>[3x]MRRFGSKFASGLASRCALACPLASAATAPAGASTTSSTSSAQKSFFKTTEMIGYVHSIDGTIATLIPAPGNPGVAYNTIIQIQVSPTTFAAGLVFNLEKDGRIGIILMDNITEVQSGQKVMATGQLLHIPVGAGVLGKVVNPLGHEVPVGLVTRSRRLLDSTLGKVDTGAPNIVSRSPVNYNLLTGFKAVDTMIPIGRGQRELIVGDRQTGKTSIAVSTIINQVRINQQILSKNAVISIYVSIGQRCSNVARIHRLLQSYGALRYTTVMAATAAEPAGLQYLAPYAGVTMGEYFMNRGRHCLCVYDDLSKQAVAYRQISLLLRRPPGREAYPGDVFYLHSRLLERAAMLSPGKGGGSVTALPIVETLSNDVTAYIVTNVISITDGQIYLDTKLFTGGQRPAVNIGLSVSRVGSSAQNAAMKGVAGKLKGILAEYRKLAADSVGGQQVQTIPMIRGARFVALFNQKQPSYFMNAIVSLYACLNGYLDDVKVQYVKFYEYLLVHRDLGIMYGTAKNKFFYMYVQELNYLIRFFTLNSPILHGELEEMLKQHTHLFLQHYQSKMNAIKSEKDVKALKNLLYSCKRAV;>MLTRFRSAVLRGAVSITGARAASTAPVADHKGRVGHVSQVIGAVVDVHFADGVPPVLTALDVVDKLGRDEPLTLEIVQHLDAHTGRCIAMQTTDLLKLKAKVVSTGGNISVPVGRETLGRIFNVLGDAIDQRGPVGEKLRMPIHAVAPKLADQAAEDAVLTT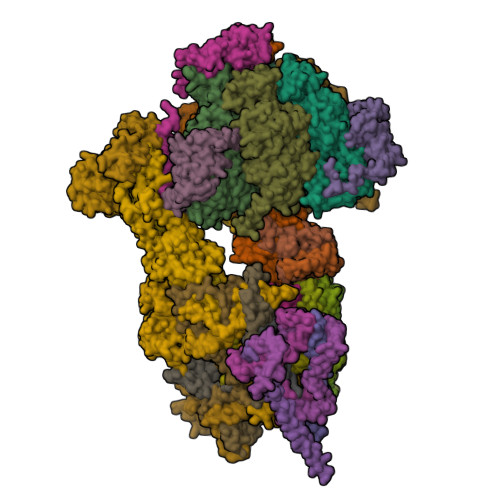GIKVIDLILPYCKGGKIGLFGGAGVGKTVIIMELINNVAKGHGGFSVFAGVGERTREGTDLYLEMMQSKVIDLKGESKCVLVYGQMNEPPGARARVAQSALTMAEYFRDVEGQDVLLFIDNIFRFTQANSEVSALLGRIPAAVGYQPTLAEDLGQLQERITSTTKGSITSVQAVYVPADDITDPAPATTFSHLDATTVLDRAVAESGIYPAVNPLECASRIMDPDVISVDHYNVAQDVVQMLTKYRELQDIIAVLGIDELSEEDKLIVDRARKLVKFLSQPFQVAEVFTGMTGHYVQLDDTIDSFSGLLMGTYDQVPEMAFYMVGGINSVLEKAKKMAEEAAELEKMRRARVAQASS[3x];> MSGKLRLYKEKLEGYNRFYSIVKTIKMVTLAKYRAAQGRIRTRDFSLRYTELAFSKPQASRDAVVAAKNALVYIPITTNRGSCGALNSNIVRCIDSVVSSKMVLMPVGKRGIDSFSKLYPDEFRYGIINDMKESMHFGYATFVIENAYEVSKDADRYQVIFNRFVSAGVQRNAVYNIPSYEKWKEDLADAASSDNQKNRYLFANALQNEEEQLIRDFFDFHAALAVLNAVGENELSEQAARLVAVEGQLTNISSLQQRTSSLYNKTRQFGITAALIEILSAMSSLEGNAMKGVRRNKFWEGAVTK;> MFRTFGRRLVSCTLPLLQSAPHDLPEGFEFMEHKVVNKDIHAPHENLETLRLTLTRQDEFLLREEPVKCVTVTGTNGEYGIYPGHAYKIVQLNPSPLTVEYTDGTTKKYFVSGGFAHINNEGSCDVNTVECTLLDDLDLAIAEKELAAQQAALGSAKDDKAKSVVEIRISVIEAVIAALKHH;> MIRRSCALLSSSWRDHGISYLKYLNVCTETLHSTVKESRRAKYERWSKPCYTAQRPDGAGGQETIDKVPIHTKDY;>[3x]MMRRVYSPVFCSVAAARFAATSAAKKYDLFGYEVDTNTAPWIEKIKKCKYYDEAGEVLVNMNVSNCPPDIATYNATLQCIYQSPSKQSTPVDNESKFCAMMDLLEEMQHRNRLKPNEESWTWVMKECVKSGQFRLGYCIQQVMETECKGCPADLVKANEANAQKAKTEGKEHPGHLSQQAGLFDVKVE;>MSAKAAPKTLHQVRNVAYFFAAWLGVQKGYIEKSANDRLWVEHQRKVRQQNVERQQALDSIKLMQQGVRATTPGQLEGVPAELQQLAEAFTK[2x];>[2x]MSSTKCAVACKIMTPLCNAASKVQARSAKKLAALTDAGIQKTISEHNANGTDAAVSSTKRYLAEQRQLFHYRVVRFFDECHYIISGEYFAQYTKVNLIWDLRFLTKLVVLFLIGTVLGRQSIFPPIDPDSPLVEALVTKVNPNY;> MFRRLSSSARAVVAARFYTPPEGLKKLYASDFENSKYPLNIVPSDSVLFAKFLYKAAEEKGNFDNILSDFQKIAAAASKLPIFWERTAVVEKIPEFKQLSEPTFFTLVWMQNNGMLELIQEVAEVYETFVNAKQKKAVAKIFVAPGGEKNVEEARRVAEELHKGLKELADYTLVLKTVVDRTIVKGFAVELAGQYVNKAEGQQKQAGRADEVDYTNLPAPKPQKTVWDDNIETEVLRKYLDGLSQYDMEEAKYGV;>MMRRLALQSSIRRATPFATPLVASTKALNPMCSAITIREASTVAISVQGLHYVGTGLAAIALAGVGLGIGTIFGNLLVACARQPNLTKMLFNYAILGFALTEAIGLFALMLAFLMLFS[10x];> MFLFFFCDLFWLRLLLCMYYCVWSRLCFIVYFNCLMLIFDFLLFCLFDLYLFVGLCLFLLLWFMLFNLYSLILYYCITYLNLYLLFCIVFLLYIAFLFLFCFLCDFFLFNNLLVGDSFMDVFFIRFLLCFLECFSLLCRCLSTFLRLFCNLLSSHFLLLMFFDFFYFIFVFFFYGVFCYWFILFIFVFCFCLLFYVFLYLLDLFAAILQLFIFCNMILQLIMDFLLFLLFV;> MLRRLGANVSNMARPMNKYAVTVSPRRHLEPMSTWYLASWAMVWYYAFFFWMPMVWTDIMVPSFVYNKLPVIHFLQEKRAEQKLRRVLDETYTEWTEELDQAHVTDAITRSLNI;> MRRVSSPNITIQSVRWISGVSPLLYFPPTTTSTTNREDQINKNTNIAIQMIKRYKGEVPPHYTRKSSATIEQVEKEIDALLGGAEKLRKTSTDDQPMDKLTLMERCLRHALWSYHKEEGRYDFDQIGRWVVYTPEDEVKLAQLKREVEAKEKLAALRKRREEEGLPGGPVPRINWPQEYSSFIDREPVVAKRIRYDTLASTTLERDEKQIESTLQQYRRASQDKRLDDLVDLLERFKPVLAREAIMQRLTIKHLEGQLGVWRYMDWCPEVRDRAELEVDITGWQWWSPLEERRLLPVRLRSVNEVREIMSKTQAKKSAEAAERNPIVTQTSTGDNARDRLLKEVLALQARINQRDEVEPSQTEQKKKAHH;> MQGSWSVLKKNCSNFFPGLLAFAQQTQEAYGIWLRIYNRQQKYGPTDFVEQSETFSPDYHKRFHSQDKNMWVDKELCTEVSQKEVARLMTYKLDMWRMAHCAGALLATGGYAIPFGLFWLANDTWVPSSFNLTGEELRAWREAQDLYRYRSAPSYLTDTKWHFDFHAYPWNETQERAWDDLFEKNDVRRDPKVVRPAAEMYDGFIKFELIRRKSLRHLCRSMNIPTFPMLARLCNGTRVRDYWNLAWCEDYMVITQRLHESMTDEELYDYAWRRYLAPYDKNLNREQLMERVEDYFEFLGPDFVAHGKAPNLVILTNYVLGYYNDPAYLEGDISELDKNDYDHLASWGKDAFLRRLEFENGPLRDQVEAHTQRLLAERAAIAKGDNAAAVEGRHTA;> MVLFSTYRSSRLVSKEFLHGPVMRFRALGEYYFQRAWNGTLNWALPGEYRLYAVMIPFIYFYHRWHNDHTLDRDHVEKAMIMRWGGTLEDVRKLSAKDQLRVRCFTDIEKLYSAYGPKDTYLQPPGDTLPGKDFYRKAGGAQAHH;> MSKQLTFISAGATAAVLQSASAIVSKVAGGRVQTKTAKEAGRHAVVVGPETPIGVHTAVTEVPKSAQDPLFSGVSTVVVRAVLPRAAPDSVQLRDALDVYASAGIDTKEEVRSATEAFKKSAEVAVGKAKAKGVKRIVLVVKQASKHNCINELFKKISTETIESAGLTTEVVGTAAVANQLIVNPESLGVVLLNDVAATEQIELAFAGVVGGVSRVYHTVEGGKISAGHSFKSVALAVAQELRELGLSSEADKVEAAASKNPRAVVSAL;> MRRTFISFSAASAAAAAPVTSTKMQTLHKLLTGEVSFKNKAPVKDCNIVHQFGENWATELSAYAKTLPAEQQKIIVRQIARVKLTRYTVAELAAYCGDGPALLDETARAANIEQGVAFVKAKGVEAFEKYVAEESTNANWKPEEAKKFIEDVKAKAK;> MVYTRWKCDRLPVFQLKLFTQEYPMHAAVGIFTIIFLWKHMSHCSEETERKYGWWAGYPYWRDPIARRNETKYKQMIINNDVDITHPKWTGCSVEQLEELSRVV;> MTKYELKMQYFDEWMIRWRKFQTESDWEIEKGRQWWRRFNMAVSGALFCGLVLYTSGTATLKRQYGLPHFFDIGVDGQAKETMLKTLTSRWRYTPQGYGRVLITGVPTYILFVTLEHYRERRRMQQYLQQNTVFGEQMRRLLSTGKIEEYLPVNIKATLPASQQAIYNY;> MLRRSSAALIRRTPVRHSGGELFVRPKLEEIPPADQCRGFFGPLNDSLKFLRLLDIKWMMNRAVAMRREYLIATPTLFTFIWMFTWKGAVIYFWGDRAPPRRMDWNTEETGRLPLGFKPTPAPL;> MLRKTPLFAMATTRKALVGNGPTFSTGGECMNTCDIQNAFPMNDRGVRSSSPFQEPNTAIYDSYLAWTYFQPMDVHIEKLPAPEAKYYQRHTKKPWDVSSTELTEIQSRKKYFQTLGYLVAFIYLYFLMPKEKSFSGLSGPDGHWIMLPKGRPELF;> MSSGFHFHDVSNDAIKGMPPSEALHKHLENAQLAHRICLAKALKAGEPPVEKCALTWGEVLIRYQAWSEYRPPFQDSVAQAKYKKYWSKKRQEEDDKNPFK;> MLRRLVPRVMMAPMGGATALCTSRGYNMLVFRDPKRRPQLSEEERAKVVVNQAEWPEEFKDFDPDDPYKNSPEIIKGMSSWNLFLWGVECAFIYQFYELVFPKSI;> MTENIEAVMSDFWSNPADHFRPNLKALTLYAERQHYVDRWLHVKERWLAPWYLPWWSPLFQLGTWYSQRSRNLFLVENHLSYRPYKFRRNDEDRNNPY;> MLLGGFVPRRFSQFNRDPCWMFFIFSVGFWLGEYPAMMIKYNARDLVYDPHRYVWSHHDDHH>MAYPYQTQGFTLDNSGRRIVVDPVTRIEGHMRCEVNIDSNNVITNAVSTGTMWRGLEVILKGRDPRDAWAFVERICGVCTGTHALTSIRAVENALGIAIPDNANCIRNMMQATLHVHDHLVHFYHLHALDWVDVVAALKADPHQTSAIAQSLSAWPLSSPGYFRDLQNRLKRFIESGQLGPFRNGYWGHPAMKLPPEANLLAVAHYLEALDFQKEIVKIHTVFGGKNPHPNWLVGGVPCAINLDETGAVGAVNMERLNLVSSIIQKARQFCEQVYLPDVLLIASYYKDWAKIGGGLSSMNLLAYGEFPDNPNDYSASNLLLPRGAIINGRFDEIHPVDLTAPDEIQEFVTHSWYTYGNGNNDKGLHPWDGLTEPQLVMGEHYKGTKTFIEQVDESAKYSWIKSPRWKGHAMEVGPLARYLIGYHQNKPEFKEPVDQLLSVLKLPKEALFSTLGRTAARALESVWAGNTLQYFFDRLMRNLKSGDTATANVTLWEPDTWPTSAKGVGFSEAPRGALGHWIKIANQKIDSYQCVVPTTWNAGPRDDKGQIGAYEAALMGTKLAVPDQPLEILRTLHSFDPCLACSTH[3x];>[3x]LENKPRTPVIWLHGLECTCCTESFIRSAHPLAKDAILSLISLDYDDTIMAAAGQQAEQALADVMREYKGNYIVAVEGNAPLNEDGMFCILAGEPFLEKLKRVSADAKAIIAWGSCASWGCVQAARPNPTKATPVHKLITDKPIIKVPGCPPIPEVMSAVITYMLAFDRIPPLDRLGRPKMFYGQRIHDKCYRRAHFDAGQFVEAWDDEGARKGYCLYKMGCKGPTTYNACSTVRWNDGVSFPIQSGHGCLGCSEDGFWDYGSFYSRATGSRSHHHHHHH

H2 oxidation (or ‘uptake’) is catalysed in S. enterica by three [NiFe]-hydrogenases encoded by the hyaABCDEF (STM1786–STM1791), hybOABCEDFG (STM3150–STM3143), and hydABCDEFGHI (STM1539–STM1531) operons. All three S. enterica H2-uptake enzymes comprise similar ‘core’ structures with a large subunit (or α-subunit) containing the [Ni–Fe–CO–2CN−] catalytic centre, and a small subunit (or β-subunit) containing three Fe–S clusters. Whereas the hya and hyb operons are up-regulated during fermentation and anaerobic respiration respectively, the hyd operon is optimally expressed under aerobic conditions. This finding led to an initial biochemical study of Hyd-5 that revealed that Hyd-5 belongs to a class of aerobically expressed ‘O2-tolerant’ hydrogenases, i.e. [NiFe]-hydrogenases, that can sustain H2 oxidation in the presence of O2. A key feature of the O2-tolerant enzymes is the special Fe–S cluster located proximal to the [NiFe] active site.

A strong promoter was placed upstream of the native hydABCDEFGHI operon on the S. enterica chromosome, and a stretch of sequence encoding the small subunit TM domain was replaced with DNA encoding an affinity tag. This allowed isolation and characterization of a water-soluble active variant of Hyd-5. The isolated Hyd-5 enzyme was subjected to size-exclusion chromatography before being concentrated and entered into crystallization experiments under standard aerobic conditions. Hyd-5 crystallized with three core hydrogenase αβ heterodimers in the asymmetric unit, and two of the three hydrogenase dimers associated with each other as an α2β2 heterotetramer. The third heterodimer in the asymmetric unit self-associates about a crystallographic 2-fold axis to produce the same α2β2 arrangement. The Hyd-5 structure also has strong feature in the electron density that would correspond to a hydrated Mg2+ ion. The Fe–S clusters are typical of an O2-tolerant hydrogenase, with a medial [3Fe–4S] cluster co-ordinated by three cysteine residues, and a distal cubane [4Fe–4S] cluster co-ordinated by three cysteines and one histidine. The special proximal [4Fe–3S] cluster of the small subunit is co-ordinated by six cysteine residues. Strikingly, however, a conserved histidine residue (His229) of the large subunit comes close to, and points directly at, the proximal [4Fe–3S] cluster. The distance between the large subunit His229 NE2 and Fe of the cluster is 3.3–3.5 Å, which is not a direct co-ordination of the metal, but certainly close enough to potentially have an effect on the properties of the cofactor. In the Hyd-5 structure, the Glu73 side chain appears to donate a hydrogen bond to the carbonyl of Pro230 in the large subunit, and this indicates that it is protonated.> AQHPPYCRNQPGKCQIPLQSLFDRATTVANYN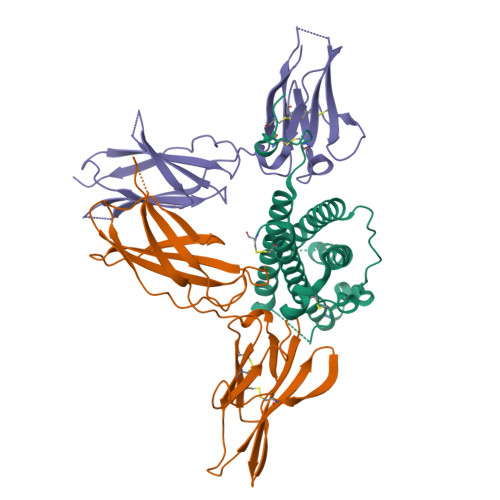SKLAGEMVNRFDEQYGQGINSESKVINCHTSSITTPNSKAEAINTEDKILFKLVISLLHSWDEPLHHAVTELANSKGTSPALLTKAQEIKEKAKVLVDGVEVIQKRIHPGEKNEPYPVWSEQSSLTSQDENVRRVAFYRLFHCLHRDSSKIYTYLRILKCRLTSCET;>QSPPGKPEIHKCRSPDKETFTCWWNPGTDGGLPTNYSLTYSKEGEKTTYECPDYKTSGPNSCFFSKQYTSIWKIYIITVNATNQMGSSSSDPLYVDVTYIVEPEPPRNLTLEVKQLKDKKTYLWVKWSPPTITDVKTGWFTMEYEIRLKPEEAEEWEIHFTGHQTQFKVFDLYPGQKYLVQTRCKPDHGYWSRWSQESSVEMPNDFTLKD[2x]> ISIGYLLVKHSQTDQEPMCPVGMNKLWSGYSLLYFEGQEKAHNQDLGLAGSCLARFSTMPFLYCNPGDVC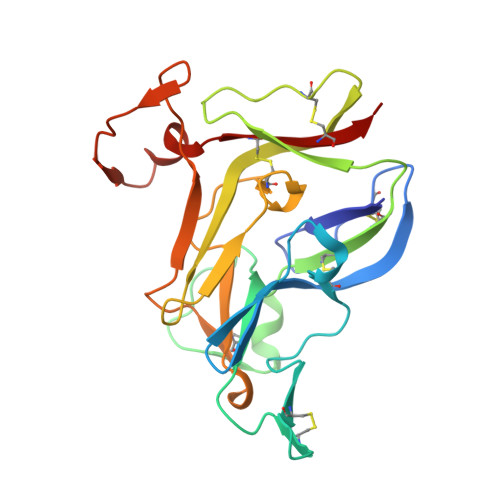YYASRNDKSYWLSTTAPLPMMPVAEEDIRPYISRCSVCEAPAVAIAVHSQDVSIPHCPAGWRSLWIGYSFLMHTAAGDEGGGQSLVSPGSCLEDFRATPFIECNGARGTCHYYANKYSFWLTTIPEQSFQGTPSADTLKAGLIRTHISRCQVCMKNL> SRDPDNIAAWYLR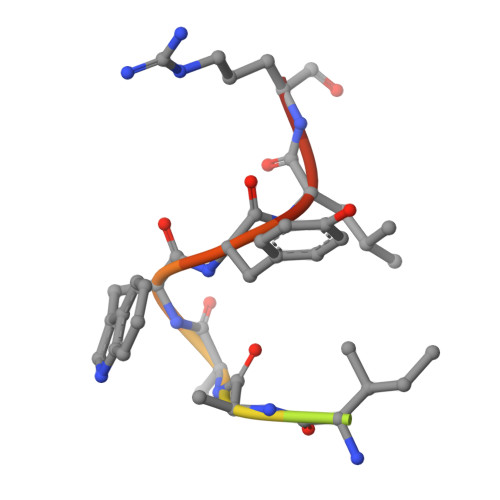S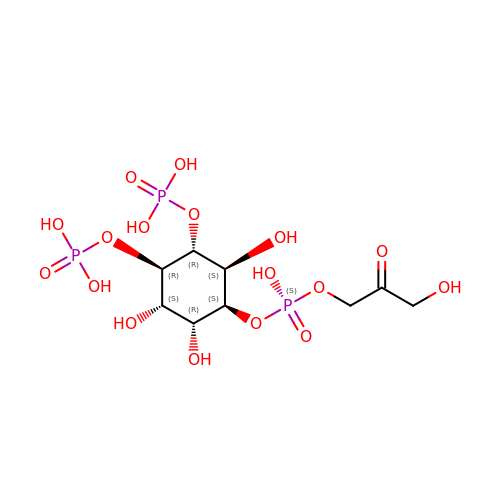L-ALPHA-GLYCEROPHOSPHO-D-MYO-INOSITOL-4,5-BIS-PHOSPHATE | C9 H19 O17 P3 | JBQPYAMQMBKZDT-WKBARDANSA-N> TEFLKPRLVDIEQVSSTHAKVTLEPLERGFGHTLGNALRRIL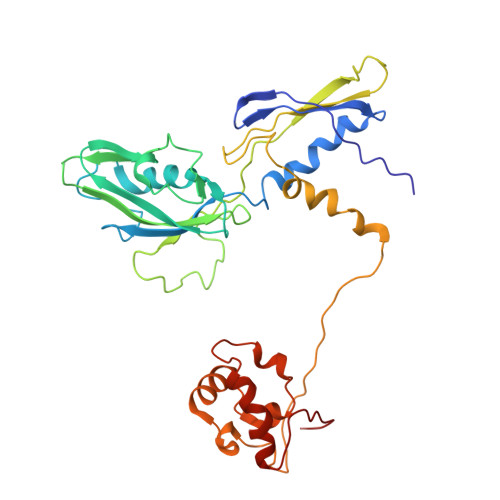LSSMPGCAVTEVEIDGVLHEYSTKEGVQEDILEILLNLKGLAVRVQGKDEVILTLNKSGIGPVTAADITHDGDVEIVKPQHVICHLTDENASISMRIKVQRGRGYVPASTRIHSEEDERPIGRLLVDACYSPVERIAYNVEAARVEQRTDLDKLVIEMETNGTIDPEEAIRRAATILAEQLEAFVDLRDVRQPEVKEEKPEFDPILLRPVDDLELTVRSANCLKAEAIHYIGDLVQRTEVELLKTPNLGKKSLTEIKDVLASRGLSLGMRLENW2-{[(1H-1,2,4-triazol-5-ylsulfanyl)acetyl]amino}thiophene-3-carboxamide 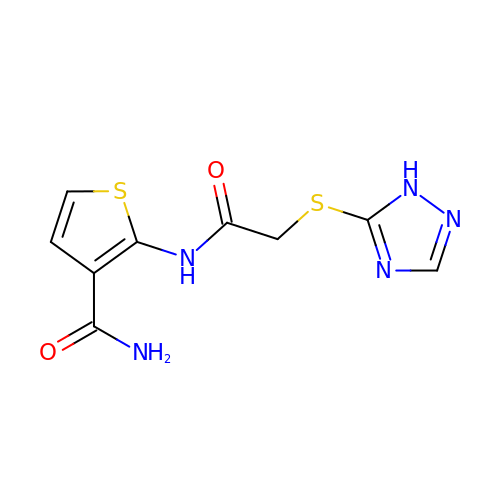| C9 H9 N5 O2 S2 | JVENGIHWHCEXOC-UHFFFAOYSA-N> MSDVAETLDPLRLPLQGERLIEASAGTGKTFTIAALYLRLLLGLGGSAAFPRPLTVEELLVVTFTEAATAELRGRIRSNIHELRIACLRETTDNPLYERLLEEIDDKAQAAQWLLLAERQMDEAAVFTIHGFCQRMLNLNAFESGMLFEQQLIEDESLLRYQACADFWRRHCYPLPREIAQVVFETWKGPQALLRDINRYL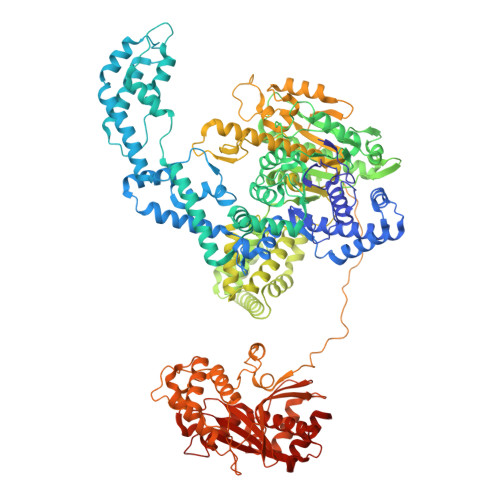QGEAPVIKAPPPDDETLASRHAQIVARIDTVKQQWRDAVGELDALIESSGIDRRKFNRSNQAKWIDKISAWAEEETNSYQLPESLEKFSQRFLEDRTKAGGETPRHPLFEAIDQLLAEPLSIRDLVITRALAEIRETVAREKRRRGELGFDDMLSRLDSALRSESGEVLAAAIRTRFPVAMIDEFQDTDPQQYRIFRRIWHHQPETALLLIGDPKQAIYAFRGADIFTYMKARSEVHAHYTLDTNWRSAPGMVNSVNKLFSQTDDAFMFREIPFIPVKSAGKNQALRFVFKGETQPAMKMWLMEGESCGVGDYQSTMAQVCAAQIRDWLQAGQRGEALLMNGDDARPVRASDISVLVRSRQEAAQVRDALTLLEIPSVYLSNRDSVFETLEAQEMLWLLQAVMTPERENTLRSALATSMMGLNALDIETLNNDEHAWDVVVEEFDGYRQIWRKRGVMPMLRALMSARNIAENLLATAGGERRLTDILHISELLQEAGTQLESEHALVRWLSQHILEPDSNASSQQMRLESDKHLVQIVTIHKSKGLEYPLVWLPFITNFRVQEQAFYHDRHSFEAVLDLNAAPESVDLAEAERLAEDLRLLYVALTRSVWHCSLGVAPLVRRRGDKKGDTDVHQSALGRLLQKGEPQDAAGLRTCIEALCDDDIAWQTAQTGDNQPWQVNDVSTAELNAKTLQRLPGDNWRVTSYSGLQQRGHGIAQDLMPRLDVDAAGVASVVEEPTLTPHQFPRGASPGTFLHSLFEDLDFTQPVDPNWVREKLELGGFESQWEPVLTEWITAVLQAPLNETGVSLSQLSARNKQVEMEFYLPISEPLIASQLDTLIRQFDPLSAGCPPLEFMQVRGMLKGFIDLVFRHEGRYYLLDYKSNWLGEDSSAYTQQAMAAAMQAHRYDLQYQLYTLALHRYLRHRIADYDYEHHFGGVIYLFLRGVDKEHPQQGIYTTRPNAGLIALMDEMFAGMTLEEA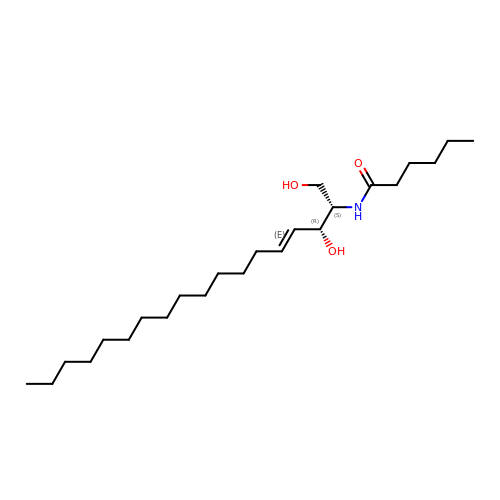N-((E,2S,3R)-1,3-DIHYDROXYOCTADEC-4-EN-2-YL)HEXANAMIDE | C24 H47 N O3 | NPRJSFWNFTXXQC-QFWQFVLDSA-N(1S,2S)-N-(7-chloro-6-{1-[(3R,4R)-4-hydroxy-3-methyloxolan-3-yl]piperidin-4-yl}isoquinolin-3-yl)-2-(1-methyl-1H-pyrazol-4-yl)cyclopropane-1-carboxamide 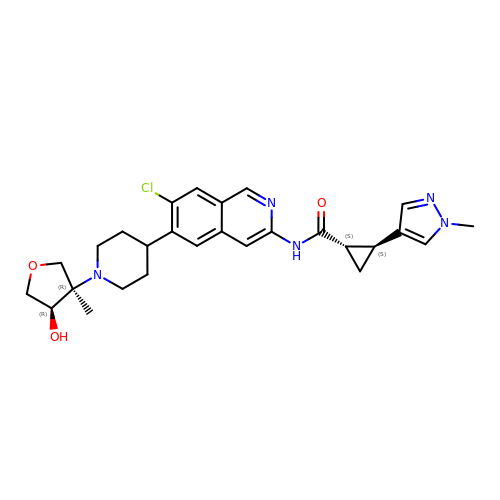| C27 H32 Cl N5 O3 | ZQNPWSJRKWOXCM-LQZFSELZSA-N> A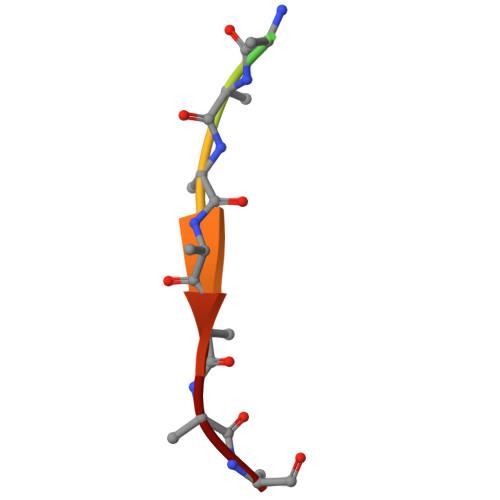AAAAAAAAA> GPGSNEATASTPVQYWQHHPEKLIFQSCDYKAFYLGSMLIKELRGTESTQDACAKMRANCQKSTEQMKKVPTIILSVSYKGVKFIDAANKNIIAEHEIRNISCAAQDPEDLSTFAYITKDLKSNHHYCHVFTAFDVNLAYEIILTLGQAFEVAYQLAL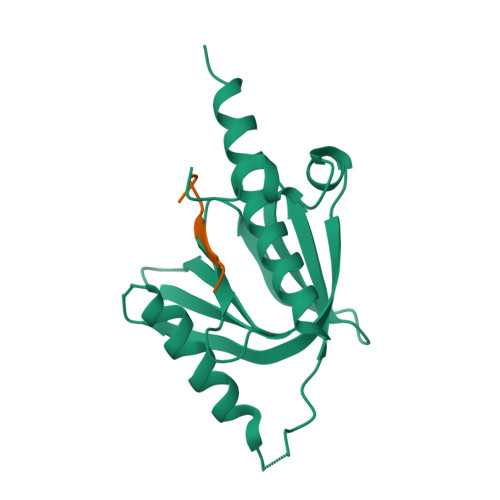QARK;> PLSFQNPLFHM> VAKLGFLFAGQGAQYVGMGKEFFDNFEESKEVFKRSSEALGIDMEELCFNDPEGLLNKTEFTQPAIITTNMAILTALDKLGVKSHISCGLSLGEYSALIHSGAINFEDGVKLVKKRGKFMQEAVAEGIGGMVAVLRMTPEQVDEIIEKSSPYGIVEGANYNSPGQIVISGELVALEKAMEFIKEVGGRAIKLPVSAPFHCSMLQPAAEKLEDELNKISINKLNGIVMSNVKGEAYLEDDNIIELLTSQVKKPVLFINDIEKMIESGV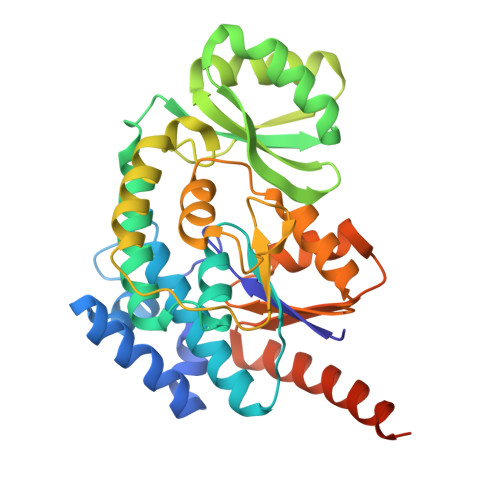DTFIEIGPGKALSGFVKKINKNVTVLNVEDLKSLEKTLSKLREMEVLAENLYFQSHHHHHHWSHPQFEK> MAYNKIPPRWLNCPRRGQPVAGRFLPLKTMLGPRYDSQVAEENRFHPSMLSNYLKSLKVKMSLLVDLTNTSRFYDRNDIEKEGIKYIKLQCKGHGECPTTENTETFIRLCERFNERSPPELIGVHCTHGFNRTGFLICAFLVEKMDWSIEAAVATFAQARPPGIYKGD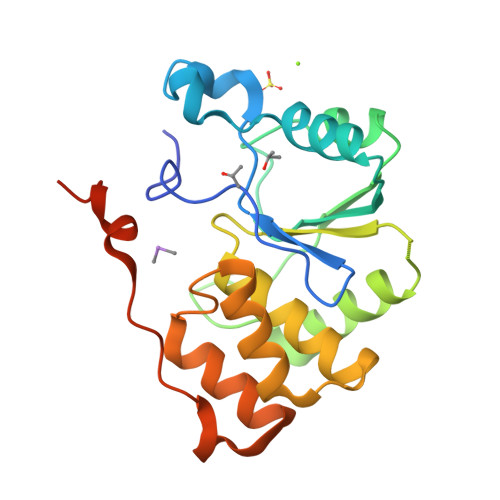YLKELFRRYGDIEEAPPPPVLPDWCFEDEDEEDEDEDGKKDS>[2x]GPGSEVPADGNAGLLAEPQIAMFCGKLNMHMNVQNGKWESDPSGTKTCIDTKEGILQYCQEVYPELQITNVVEANQPVTIQNWCKRGWKQCNGHPHIVVPYRCLVGEFVSDALLVPDKCKLLHQERMDVCETHLHWHTVAKESCSEKSMNLHDYG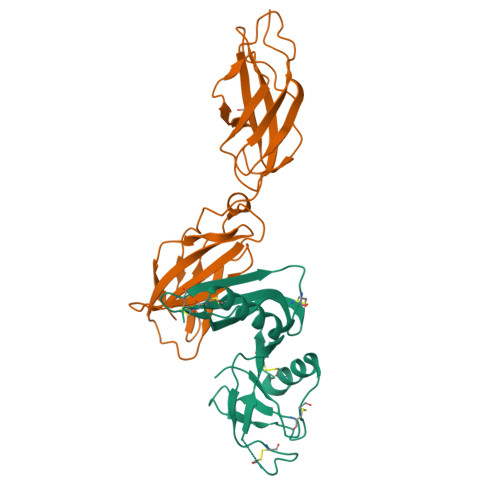MLLPCGIDKFRGVEFVCCPLAEESDNLDS;>GSTGSPPGPPEDVTIDEITDTTAQLSWRPGADNHSPITMYVVQARTPFSVGWQAVSTVPEVIDGKTFTATVVGLNPWVEYEFRVVAANLIGIGEPSRPSENRRTEEALPEVTPANVSGGGGSKSELVITWETVPEELQNGGGFGYVVAFRPFGTISWMQTVVASPDASRYVFRNESLPPFSPYEVKVGVYNNKGEGSFSPVTVVYSAEEEPTRAPITVLARSLSATDIEISWAPPRENQHKGRIQGYEVRCWRHDEKEENARKIRTVGNQTSAKVTNLQGNALYHLAVKAYNTAGTGPSSAMVNVTTKK[2x]> EASLL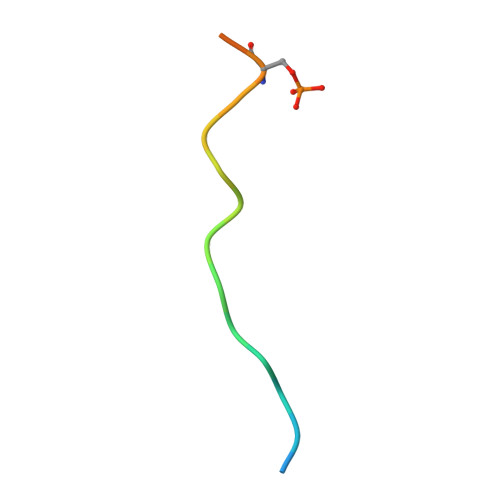SFEKLDRASPDLWPE4-benzyl-3-[(2-chlorobenzyl)sulfanyl]-5-thiophen-2-yl-4H-1,2,4-triazole | C20 H16 Cl N3 S2 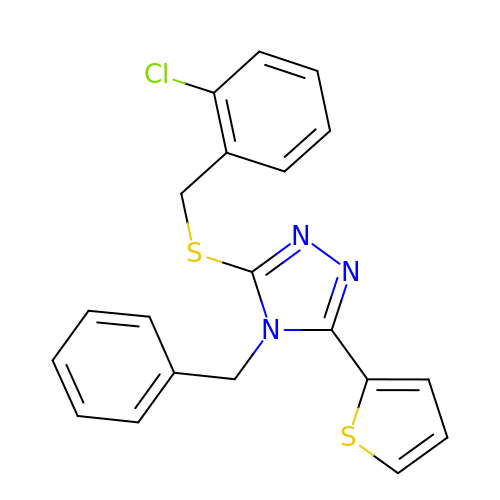| FMDVHVQWAJPVKM-UHFFFAOYSA-N>[2x]SSATPIVQFQGESNCLKCFRYRLNDKHRHLFDLISSTWHWASP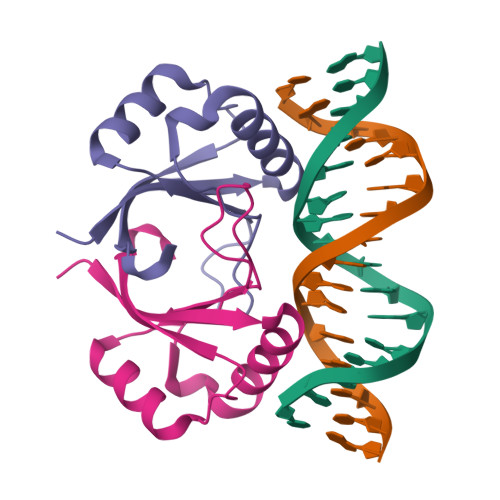KAPHKHAIVTVTYHSEEQRQQFLNVVKIPPTIRHKLGFMSMHLL>[10x]MGLEDKVSKQLESKGIKFEYEEWKVPYSNNQQNY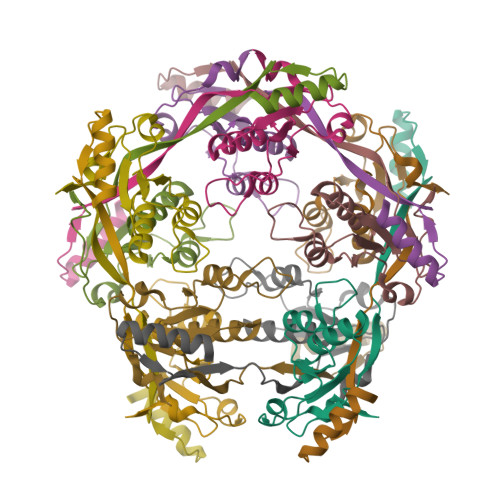SSHTYTPDFLLPNGIFVETKGLWESDDRKKHLLIREQHPELDIRIVFSSSRTKLYKGSPTSYGEFCEKHGIKFADKLIPAEWIKEPKKEVPFDRLKRK> MGAQVSTQKTGAHETGLNASGNSVIHYTNINYYKDAASNSANRQDFT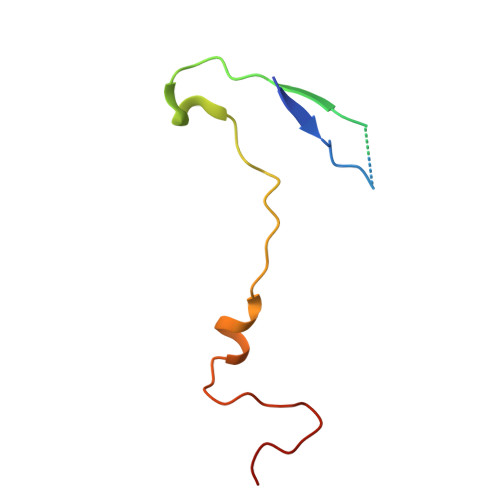QDPGKFTEPVKDIMVKTMPALN>MAHHHHHHHRSADPDPGGPTTAENLSKEAVRFY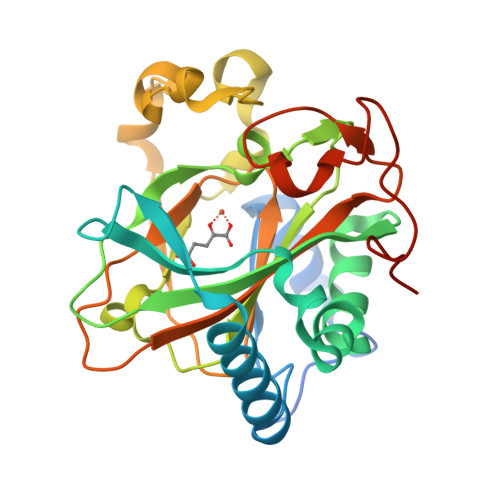REQGYVHIPRVLSETEVTAFRAACEEVLEKEGREIWGAGEDEVQVHYVAQAWQKHPELRSLVLHPEISGIALRLAGAPLRVYSSDILVKEPKRTLPTLVHDDETGLPLNELSATLTAWIALTDVPVERGCMSYVPGSHLRAREDRQEHMTSFAEFRDLADVWPDYPWQPRVAVPVRAGDVVFHHCRTVHMAEANTSDSVRMAHGVVYMDADATYRPGVQDGHLSRLSPGDPLEGELFPLVTAGTRQ[6x]>MALLERILARDNLITALKRVEANQGAPGIDGVSTDQLRDYIRAHWSTIHAQLLAGTYRPAPVRRVEIPKPGGGTRQLGIPTVVDRLIQQAILQELTPIFDPDFSSSSFGFRPGRNAHDAVRQAQGYIQEGYRYVVDMDLEKFFDRVNHDILMSRVARKVKDKRVLKLIRAYLQAGVMIEGVKVQTEEGTPQGGPLSPLLANILLDDLDKELEKRGLKFCRYADDCNIYVKSLRAGQRVKQSIQRFLEKTLKLKVNEEKSAVDRPWKRAFLGFSFTPERKARIRLAPRSIQRLKQRIRQLTNPNWSISMPERIHRVNQYVMGWIGYFRLVETPSVLQTIEGWIRRRLRLCQWLQWKRVRTRIRELRALGLKETAVMEIANTRKGAWRTTKTPQLHQALGKTYWTA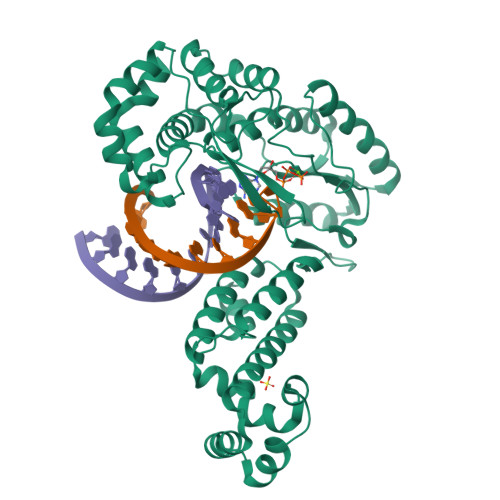QGLKSLTQRYFELRQGHHHHHHHH[2x]> ECLPGSSPCTDALT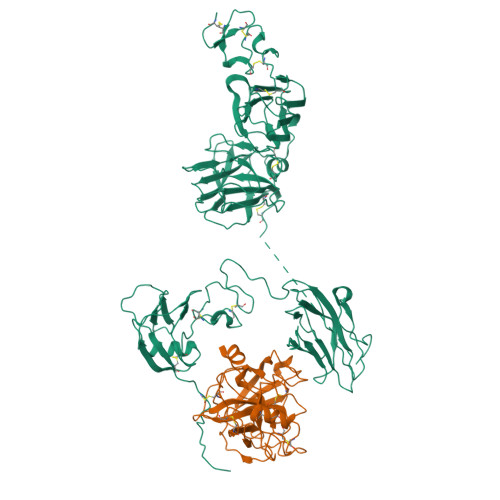CIKADLFCDGEVNCPDGSDEDNKMCATVCDGRFLLTGSSGSFQATHYPKPSETSVVCQWIIRVNQGLSIKLSFDDFNTYYTDILDIYEGVGSSKILRASIWETNPGTIRIFSNQVTATFLIESDESDYVGFNATYTAFNSSELNNYEKINCNFEDGFCFWVQDLNDDNEWERIQGSTFSPFTGPNFDHTFGNASGFYISTPTGPGGRQERVGLLSLPLDPTLEPACLSFWYHMYGENVHKLSINISNDQNMEKTVFQKEGNYGDNWNYGQVTLNETVKFKVAFNAFKNKILSDIALDDISLTYGICNGSLYPEPTLVPTPPPELPTDCGGPFELWEPNTTFSSTNFPNSYPNLAFCVWILNAQKGKNIQLHFQEFDLENINDVVEIRDGEEADSLLLAVYTGPGPVKDVFSTTNRMTVLLITNDVLARGGFKANFTTGYHLGIPEPCKADHFQCKNGECVPLVNLCDGHLHCEDGSDEADCVRFFNGTTNNNGLVRFRIQSIWHTACAENWTTQISNDVCQLLGLGSGNSSKPIFPTDGGPFVKLNTAPDGHLILTPSQQCLQDSLIRLQCNHKSCGKKLAAQDITPK;> IVGGSNAKEGAWPWVVGLYYGGRLLCGASLVSSDWLVSAAHCVYGRNLEPSKWTAILGLHMKSNLTSPQTVPRLIDEIVINPHYNRRRKDNDIAMMHLEFKVNYTDYIQPICLPEENQVFPPGRNCSIAGWGTVVYQGTTANILQEADVPLLSNERCQQQMPEYNITENMICAGYEEGGIDSCQGDSGGPLMCQENNRWFLAGVTSFGYKCALPNRPGVYARVSRFTEWIQSFLH> MLSYTSTLLRVFNRKNKAPQRMSNFTKVTNLNKAEKVKIETVDGDVVKGRGRVHRRSHSGLKDAIEEMEHPAIWLWYPWRKNPEPPTPFMPSQRALKNIHGAIFANLSPIQKKKQEQMLYGVNIPETRVMRFEQQHPLLSTALTQLDGQPKGFPFWYKKYPTRRHAYEQRFSVPTEMLEGYNDSIKKAFSMSMMTIQEKQFAQEAMYMERYAEHDFDTTSPAVLAVKRALKVRVLRNHLLTNPHNNIVKTILANTERKLNHTLRRLRKVDFKRYWEIIRDHDVQDVLQPPNLVTYRQGSYWRYDWNAGLAISTQLADVLDPRGLNGCVETGRSRSEVARDLGLSYTRPLQENEKKQLSEQAVYYERLAKFKMEQPEAARAQERERFVRKF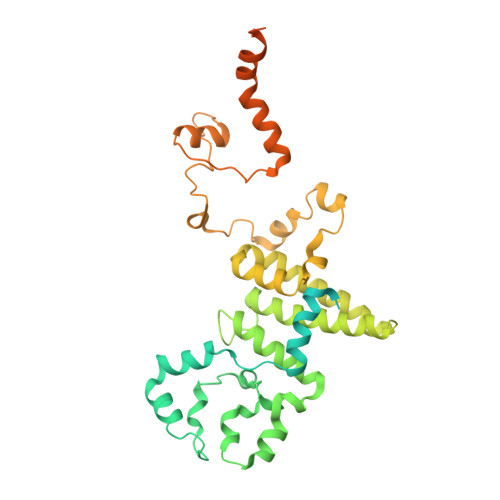SGMFLKLDMKSGVPDFPSTYRKLLGTQVARWSSKRHGPM>[2x]MTDQGLEGSNPVDLSKHPSGIVPTLQNIVSTVNLDCKLDLKAIALQARNAEYNPKRFAAVIMRIREPKTTALIF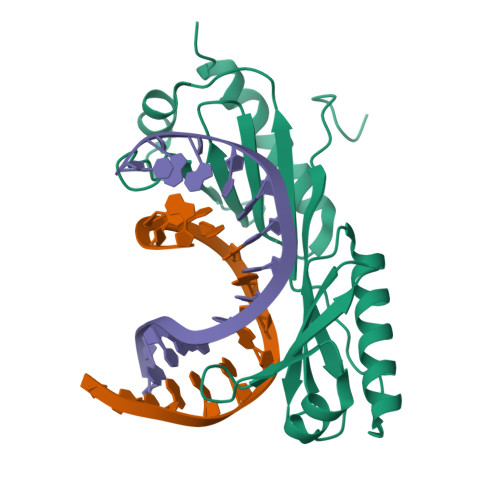ASGKMVCTGAKSEDFSKMAARKYARIVQKLGFPAKFKDFKIQNIVGSCDVKFPIRLEGLAYSHAAFSSYEPELFPGLIYRMKVPKIVLLIFVSGKIVITGAKMRDETYKAFENIYPVLSEFRKIQQ>HMVKLGKLQYSMDYDFQKGELTVNV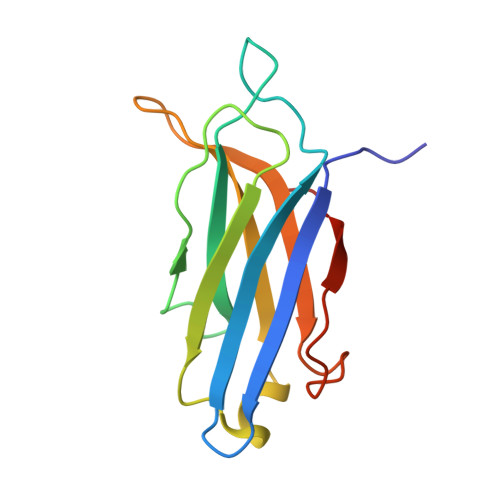IQAADLPGMDMSGTSDPYVKVYLMPDKKKKFETKVHRKTLNPVFNESFTFKNVPYADITGKTLIFAIYDFDRFSKHDQIGQVQVPMNSIDLGSVVEEWRDLTSPDN[2x]> MGAVMGTFSSLQTKQRRPSKDKIEDELEMTMVCHRPEGLEQLEAQTNFTKRELQVLYRGFKNECPSGVVNEDTFKQIYAQFFPHGDASTYAHYLFNAFDTTQTGSVKFEDFVTALSILLRGTVHEKLRWTFNLYDINKDGYINKEEMMDIVKAIYDMMGKYTYPVLKEDTPRQHVDVFFQKMDKNKDG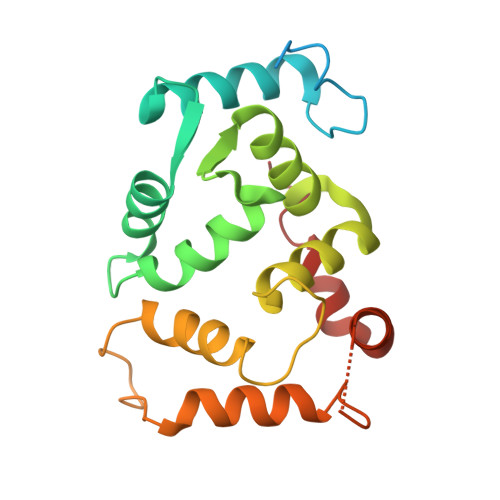IVTLDEFLESCQEDDNIMRSLQLFQNVM> NPV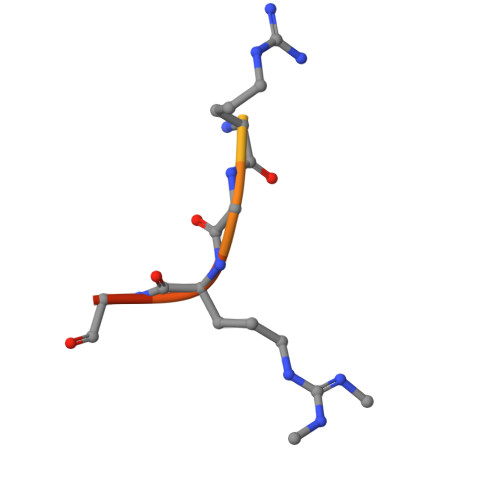IARGRGRGRK> GAKEYTNPKEGQLATTVSVKNNESTTPVRLLSKDTQGVEVTDTVSYSDLVGGKVYELTGTLMQIKADGSTEAIASASKEVTAETSGKGTWELTFAPQNLKAGEKYVVYEVAKSK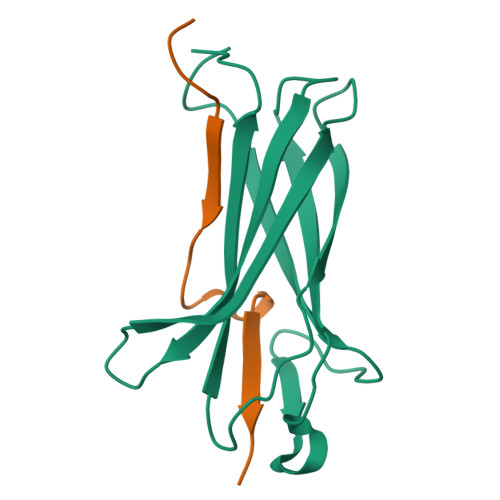ENLVDSNKDDESHG;> GDTKHEVRHENPQDEAQTIVVNK>KYRVR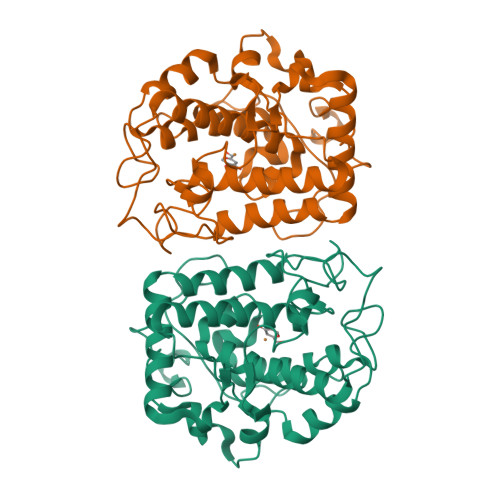KNVLHLTDTEKRDFVRTVLILKEKGIYDRYIAWHGAAGKFHTPPGSDRNAAHMSSAFLPWHREYLLRFERDLQSINPEVTLPYWEWETDAQMQDPSQSQIWSADFMGGNGNPIKDFIVDTGPFAAGRWTTIDEQGNPSGGLKRNFGATKEAPTLPTRDDVLNALKITQYDTPPWDMTSQNSFRNQLEGFINGPQLHNRVHRWVGGQMGVVPTAPNDPVFFLHHANVDRIWAVWQIIHRNQNYQPMKNGPFGQNFRDPMYPWNTTPEDVMNHRKLGYVYDIEL[2x]Toll-like receptors (TLRs) are highly conserved and crucial components of the innate immune system. Particularly, human TLR8 mediates antiviral immunity by recognizing ssRNA viruses. Particularly, TLR8 also plays an important role in the antiviral immune response through recognition of viral RNA in endocytic compartments. Previous reports have shown a two-site activation mechanism for TLR8 with ssRNA degradation products.

The efforts described herein culminate in the fortuitous discovery of a tetrasubstituted imidazole CU-CPD107 which inhibits R848-induced TLR8 signaling. Aiming to further understand the molecular mechanism of this unexpected, unique, and dichotomous behavior of CU-CPD107, we successfully obtained the crystal structure of the TLR8/CU-CPD107 complex. CU-CPD107 utilized hydrogen bonds with A518* and V520*. This newly identified compound CU-CPD107 inhibited TLR8 signaling via stabilizing its resting state which was the same mechanism with the first TLR8-specific inhibitor CU-CPT8m we have reported previously. The distances between the C termini of the two protomers of TLR8 dimer (TLR8/CU-CPD107, 50 Å) was similar to that of the unliganded dimer (51 Å). Superimposition of the TLR8 structure complexed with CU-CPD107 onto the corresponding unliganded TLR8 segment (residues 32–816) produced a root-mean-square deviation (RMSD) value of 1.2 Å. First, CU-CPD107 (100 µM) alone was titrated into purified TLR8 (10 µM), with no detectable change in heat observed; R848 (100 µM) alone was titrated into TLR8 (10 µM) with an observed Kd of 35.7 nM. For comparison, R848 (100 µM) was titrated into TLR8 protein (10 µM) premixed with CU-CPD107 (100 µM), with no heat change observed. These results indicated that CU-CPD107 hindered R848 binding to TLR8, in agreement with the inhibition observed previously. Therefore, we rationalized that ssRNA converts TLR8 to its activated conformation, and CU-CPD107 binds to the secondary site instead of uridine.

>[2x]RSPWEENFSRSYPCDEKKQNDSVIAECSNRRLQEVPQTVGKYVTELDLSDNFITHITNESFQGLQNLTKINLNHNPNVQHQNGNPGIQSNGLNITDGAFLNLKNLRELLLEDNQLPQIPSGLPESLTELSLIQNNIYNITKEGISRLINLKNLYLAWNCYFNKVCEKTNIEDGVFETLTNLELLSLSFNSLSHVPPKLPSSLRKLFLSNTQIKYISEEDFKGLINLTLLDLSGNCPRCFNAPFPCVPCDGGASINIDRFAFQNLTQLRYLNLSSTSLRKINAAWFKNMPHLKVLDLEFNYLVGEIASGAFLTMLPRLEILDLSFNYIKGSYPQHINISRNFSKLLSLRALHLRGYVFQELREDDFQPLMQLPNLSTINLGINFIKQIDFKLFQNFSNLEIIYLSENRISPLVKDTRQSYANSSSFQRHIRKRRSTDFEFDPHSNFYHFTRPLIKPQCAAYGKALDLSLNSIFFIGPNQFENLPDIACLNLSANSNAQVLSGTEFSAIPHVKYLDLTNNRLDFDNASALTELSDLEVLDLSYNSHYFRIAGVTHHLEFIQNFTNLKVLNLSHNNIYTLTDKYNLESKSLVELVFSGNRLDILWNDDDNRYISIFKGLKNLTRLDLSLNRLKHIPNEAFLNLPASLTELHINDNMLKFFNWTLLQQFPRLELLDLRGNKLLFLTDSLSDFTSSLRTLLLSHNRISHLPSGFLSEVSSLKHLDLSSNLLKTINKSALETKTTTKLSMLELHGNPFECTCDIGDFRRWMDEHLNVKIPRLVDVICASPGDQRGKSIVSLELTTCVSDVTEFLVPR>[2x]NAKGNYCKRTPLYIDFKEIGWDSWIIAPPGYEAYECRGVCNYPLAEHLTPTKHAIIQALVHLKNSQKASKACCVPTKLEPISILYLDKGVVTYKFKYEGMAVSECGCR;>[2x]GSQNQERLCAFKDPYQQDLGIGESRISHENGTILCSKGSTCYGLWEKSKGDINLVKQGCWSHIGDPQECHYEECVVTTTPPSIQNGTYRFCCCSTDLCNVNFTENFPPPDTTPLSPPHSFNRDET

The TGF-β ligands are dimers and initiate signal transduction by forming a signalling complex with two copies of a type I receptor and two copies of a type II receptor; all are single-pass transmembrane proteins containing a small extracellular ligand-binding domain (ECD) and an intracellular kinase domain (ICD). Upon signalling complex formation, the constitutively active type II receptor phosphorylates and activates the type I receptor; subsequently the type I receptor phosphorylates Smad1/5 or Smad2/3 to regulate transcriptional responses. For example, ActRIIA/B bind to and mediate the signalling from both activin ligands and some BMP ligands, whereas BMPRII is the low-affinity type II receptor for over 15 BMP ligands. Of note, BMPRII is particularly highly expressed in lung vascular endothelial cells, where it mediates the signalling from circulating BMP9 and BMP10.

We solved crystal structures of the BMPRII binary complex with BMP10 in two different crystal forms, at 1.48 Å and 2.4 Å, respectively. In the 1.48 Å structure, the asymmetric unit contains one BMP10 dimer with two copies of BMPRII. Using the chain identities to name the seven complexes, they are complexes AC and BD, complex AB and complexes AI, BJ, CK and DL from the ternary complexes. Slight variations in this region among the seven complexes include the lengths of the H-bonds, missing the interaction between BMPRII S86 and BMP10 S398 in complex BJ and AI, and complexes BD, DL, CK, BJ and AI have an additional H-bond between BMPRII K81 and the mainchain of BMP10 V407. Of note, the interaction between K81 and V407 is also present in complex AC, but instead of a direct H-bond, the interaction is mediated by two water molecules. Additional water-mediated interactions between BMP10 and BMPRII are present only in complex AC in this region. The third area is between the A-loop and the F3-loop and is different among different complexes. In complex AC, this region makes significant contact with BMP10 (orange oval), with many direct and water-mediated H-bonds. Interestingly, 5 out of 15 residues with alternate conformations in complex AC are at this area, suggesting that the conformation in this region is highly flexible. Many water-mediated H-bonds are clearly visible in complex AC from the 1.48 Å structure.> APTSSSTKKTQLQLEHLLLDLQMILNGINNYKNPKLTRMLTFKFYMPKKATELKHLQCLEE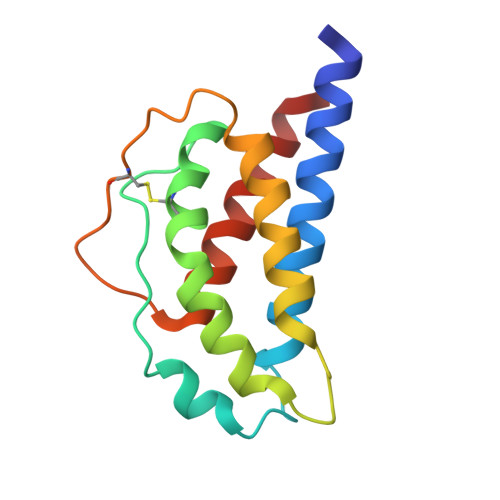ELKPLEEVLNLAQSKNFHLRPRDLISNINVIVLELKGSETTFMCEYADETATIVEFLNRWITFAQSIISTLT4-methylbenzene-1,2-dicarboxylic acid | C9 H8 O4 | 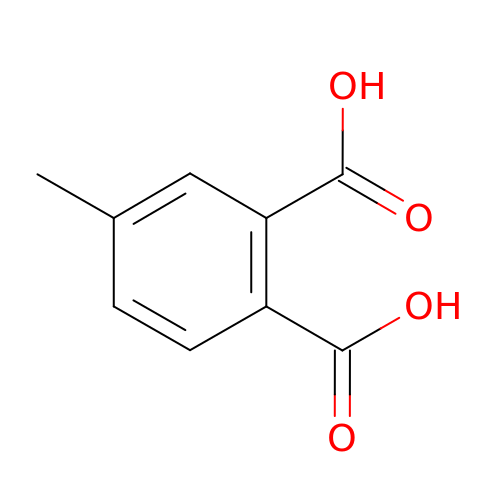CWJJAFQCTXFSTA-UHFFFAOYSA-N>[2x]MNYWWVSQKQTFKQEFEGGYMWSPKENKNGTQSHYYNNMTLVQPGDVVFSFANGLILSVGIARSHAYSYNKPTEFGVAGADWANDGWKIDLEYHLVENKIRPKAHIDFIRPYLPQKYSPLQDNGNGNQAYLFSVPHELASKVVELIGSEAEEVIFGFADTTEITTTADAIECQISNDASIDETEKHQLVKSRRGQGIFRSRLEQVESRCRVTGVQLKNHLIASHIKPWAVSNNQERLDGHNGLLLAPHVDHLFDKGFISFEDNGEMIVSEKLNLDVLKAWSISQGNYGYFSKQQQEYMCYHRENVFKKL

Modification dependent restriction endonucleases (MDREs) specifically target DNA that is modified, and are non-toxic to a host with non-modified DNA. Many modification-dependent restriction endonucleases (MDREs) are fusions of a PUA superfamily modification sensor domain and a nuclease catalytic domain. EVE domains belong to the PUA superfamily, and are present in MDREs in combination with HNH nuclease domains. In all crystal structures, VcaM4I protomers have the predicted two domain architecture, with N-terminal domains of the PUA superfamily (residues 1–147), linker helices (148–178), and C-terminal HNH domains (residues 179–309).

The crystal form without DNA was phased experimentally. Except for the weaker diffracting crystals of VcaM4I with dsDNA, the resolution of the data reached around 1.5 Å. Although crystals without DNA, with ssDNA, and with dsDNA grew in different space groups, the protein conformation was remarkably similar in all structures, with the exception of two loops in proximity of the DNA (residues 24–34 and 72–84). In all crystal forms, the protomers dimerize via the HNH domains. The extensive interface area of 2000 Å2 (equivalent to 4000 Å2 of buried surface) and the classification of the interface as stable by the PDBePISA server suggest that the dimerization mode in the crystals is relevant in solution. The DNA binding site of the C-terminal HNH domains is consistently empty in all structures. The dimer of HNH domains alone is crescent-shaped and could accommodate dsDNA (∼20 Å in diameter). The VcaM4I alone and with 11-mer duplex generated scattering profiles that indicated ‘compact’ structures judging from the Kratky plot. At low concentration, the scattering data for VcaM4I and its complex with dsDNA were well modelled by the crystallographic structures (for the enzyme alone, with dsDNA bound to one EVE domain, or the mixture model).>MGSSHHHHHHSSGRENLYFQGHMTLSSAPILITGASQRVGLHCALRLLEHGHRVIISYRTEHASVTELRQAGAVALYGDFSCETGIMAFIDLLKTQTSSLRAVVHNASEWLAETPGEEADNFTRMFSVHMLAPYLINLHCEPLLTASEVADI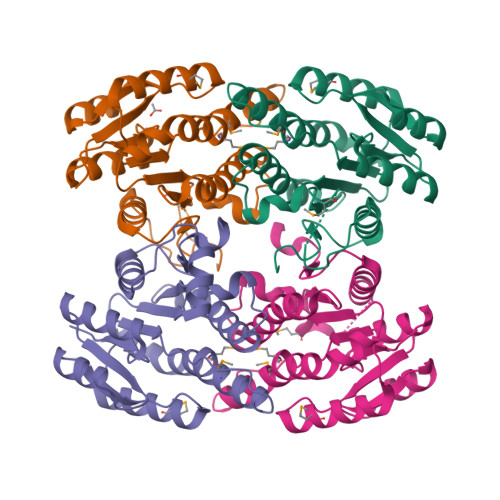VHISDDVTRKGSSKHIAYCATKAGLESLTLSFAARFAPLVKVNGIAPALLMFQPKDDAAYRANALAKSALGIEPGAEVIYQSLRYLLDSTYVTGTTLTVNGGRHVKGS[4x]>[3x]MKVNNTIVVSIGQAGNQIAASFWKTVCLEHGIDPLTGQTAPGVAPRGNWSSFFSKLGESSSGSYVPRAIMVDLEPSVIDNVKATSGSLFNPANLISRTEGAGGNFAVGYLGAGREVLPEVMSRLDYEIDKCDNVGGIIVLHAIGGGTGSGFGALLIESLKEKYGEIPVLSCAVLPSPQVSSVVTEPYNTVFALNTLRRSADACLIFDNEALFDLAHRKWNIESPTVDDLNLLITEALAGITASMRFSGFLTVEISLRELLTNLVPQPSLHFLMCAFAPLTPPDGSDGEELGIEEMIKSLFDNGSVFAACSPMEGRFLSTAVLYRGIMEDKPLADAALAAMREKLPLTYWIPTAFKIGYVEQPGISHRKSMVLLANNTEIARVLDRICHNFDKLWQRKAFANWYLNEGMSEEQINVLRASAQELVQSYQVAEESGAKAKVQDSAGDTGMRAAAAGVSDDARGSMSLRDLVDRRR;>[3x]MREILSIHVGQCGNQIADSFWRLALREHGLTEAGTLKEGSNAAANSNMEVFFHKVRDGKYVPRAVLVDLEPGVIARIEGGDMSQLFDESSIVRKIPGAANNWARGYNVEGEKVIDQIMNVIDSAVEKTKGLQGFLMTHSIGGGSGSGLGSLILERLRQAYPKKRIFTFSVVPSPLISDSAVEPYNAILTLQRILDNADGAVLLDNEALFRIAKAKLNRSPNYMDLNNIIALIVSSVTASLRFPGKLNTDLSEFVTNLVPFPGNHFLTASFAPMRGAGQEGQVRTNFPDLARETFAQDNFTAAIDWQQGVYLAASALFRGDVKAKDVDENMATIRKSLNYASYMPASGGLKLGYAETAPEGFASSGLALVNHTGIAAVFERLIAQFDIMFDNHAYTHWYENAGVSRDMMAKARNQIATLAQSYRDAS

Many protein filaments function through dynamic cycles of assembly and disassembly, characteristically using energy released through inbuilt nucleotide hydrolysis activity to perform work by pushing and pulling other molecules around. These dynamic filaments have been termed cytomotive, to distinguish them among the wider class of cytoskeletal filaments that perform organizing functions (itself a subset of all filament-forming proteins). So far, we know of only two protein families that form cytomotive filaments and have inbuilt nucleotide hydrolysis activity—the actin and tubulin superfamilies. Overall, however, the picture is clear: The tubulin superfamily, much like the actin superfamily, appears to have a shared subunit conformational switch upon polymerization.

We thus used a different system of reduced complexity: bacterial tubulin A/B (BtubAB). Prosthecobacter dejongeii BtubAB heterodimers form four-stranded (4pf) mini-MTs, which exhibit dynamic instability and treadmilling. We designed a mutant of BtubAB, intended to decouple longitudinal polymerization from lateral assembly interactions by introducing multiple mutations into the M-loop because lateral interactions are exclusively via the “MT” M-loop of BtubA. We termed this mutant BtubA*B (BtubA*: R284G, K286D, and F287G). Right: Single protofilament/1pf polymers formed by BtubA*B M-loop mutant (BtubA*: R284G, K286D, and F287G). Using cryo-EM, we resolved a 3.5-Å reconstruction of single protofilaments of BtubA*B protein polymerized with GMPCPP. Comparison of the 1pf model built into the reconstructed density with the previously determined 4pf mini-MT wild-type (WT) structure revealed that the 1pf and 4pf polymer structures were essentially identical. Our explorations of simpler-than-MT tubulin systems therefore appeared to confirm the straightforward conclusion that the conformation changes seen within eukaryotic tubulin heterodimers upon polymerization are not determined by the multistranded nature of MTs. Using three different systems also strengthened the case that the within-subunit conformation changes are shared between diverse tubulin superfamily members.>[2x]MDVNMKLTGRIMDAAKEVDHTCRSSTGVPRDMLHRYAE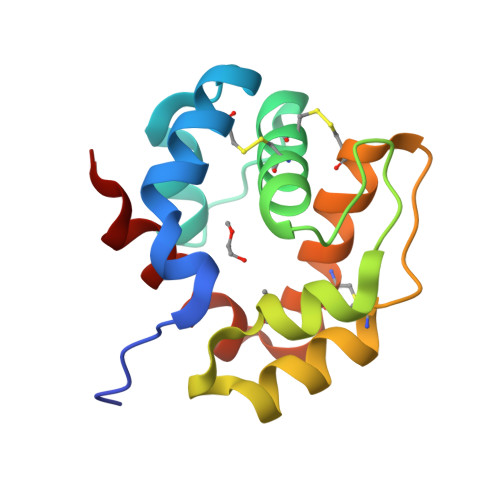GQTVDDDDFKCYLKCIMVEFNSLSDDGVFVLEEELENVPPEIKEEGHRVVHSCKHINHDEACETAYQIHQCYKQSDPELYSLVVRAFDATIGD>[5x]MTQELGNANFENFIGATEGFSEIAYQFTSHILTLGYAVMLAGLLYFILTIKNVDKKFQMSNIL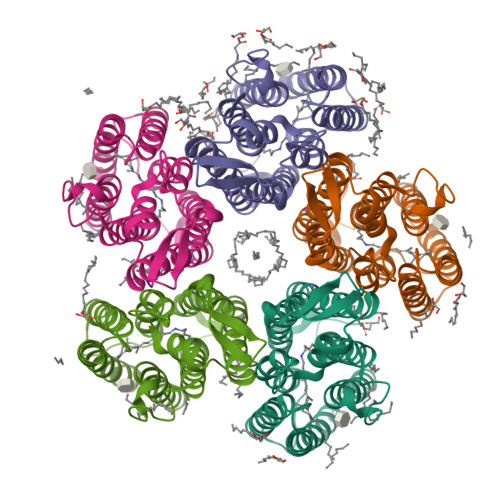SAVVMVSAFLLLYAQAQNWTSSFTFNEEVGRYFLDPSGDLFNNGYRYLNWLIDVPMLLFQILFVVSLTTSKFSSVRNQFWFSGAMMIITGYIGQFYEVSNLTAFLVWGAISSAFFFHILWVMKKVINEGKEGISPAGQKILSNIWILFLISWTLYPGAYLMPYLTGVDGFLYSEDGVMARQLVYTIADVSAKVIYGVLLGNLAITLSKNKELVEANSLEHHHHHH> GPAGLVEGQNYTVLANPIPQQQAGKVE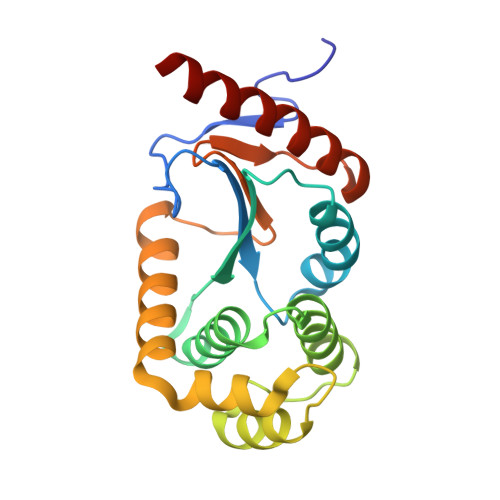VLEFFGYFCPHCAHLEPVLSKHAKSFKDDMYLRTEHVVWQKEMLTLARLAAAVDMAAADSKDVANSHIFDAMVNQKIKLQNPEVLKKWLGEQTAFDGKKVLAAYESPESQARADKMQELTETFQIDGTPTVIVGGKYKVEFADWESGMNTIDLLADKVREEQKAAQ> KET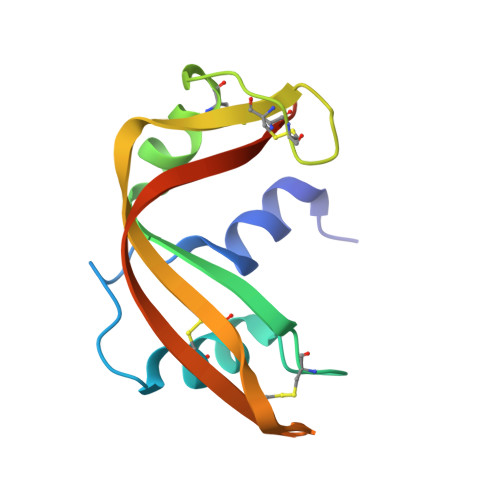AAAKFERQHMDSSTSAASSSNYCNQMMKSRNLTKDRCKPVNTFVHESLADVQAVCSQKNVACKNGQTNCYQSYSTMSITDCRETGSSKYPNCAYKTTQANKHIIVACEGNPYVPV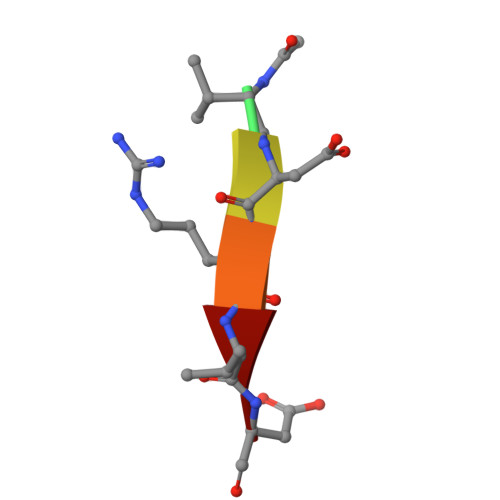> XVDRVD> MQIELSTCFFLCLLPFCFSATRRYYLGAVELSWDYMQSDLGELHVD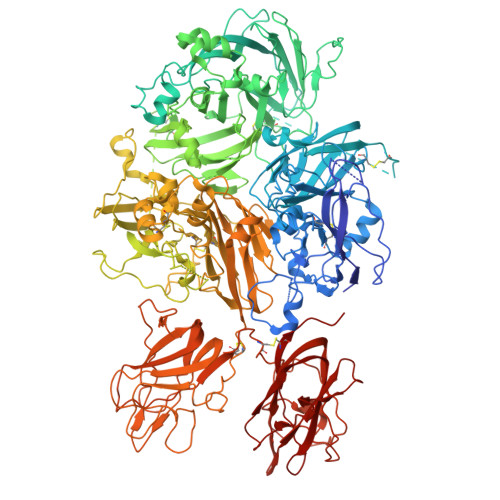TRFPPRVPKSFPFNTSVVYKKTLFVEFTDHLFNIAKPRPPWMGLLGPTIQAEVYDTVVITLKNMASHPVSLHAVGVSYWKASEGAEYDDQTSQREKEDDKVFPGGSHTYVWQVLKENGPMASDPPCLTYSYLSHVDLVKDLNSGLIGALLVCREGSLAKEKTQTLHKFILLFAVFDEGKSWHSETNNSLTQDRDAASARAQPKMHTVNGYVNRSLPGLIGCHRKSVYWHVIGMGTTPEVHSIFLEGHTFLVRNHRQASLEISPITFLTAQTLLMDLGQFLLFCHISSHQHDGMEAYVKVDSCPEEPQLRMKNNEEAEDYDDDLTDSEMDVVRFDDDNSPPFIQIRSVAKKHPKTWVHYIAAEEEDWDYAPLVLAPDDRSYKSLYLNNGPQRIGRKYKKVRFMAYTDETFKTREAIQHESGILGPLLYGEVGDTLLIIFKNQASRPYNIYPHGITDVRPLHSGRLPKGVKHLKDMPILPGEIFKYKWTVTVEDGPTKSDPRCLTRYYSSFVNLERDLASGLIGPLLICYKESVDQRGNQMMSDKRNVILFSVFDENRSWYLTENIQRFLPNPAGVQPEDPEFQASNIMHSINGYVFDSLQLSVCLHEVAYWYILSVGAQTDFLSVFFSGYTFKHKMVYEDTLTLFPFSGETVFMSMENPGLWILGCHNSDFRNRGMTALLKVSSCDKNTGDYYEDSYEDIPAYLLSKNNVIEPRSFSQNPPVLKRHQREITRTTLQPDEEKIDYDDTFSVEMKKEDFDIYGEDENQSPRSFQKKTRHYFIAAVERLWDYGMSSSPHVLRNRAQSGSVPQFKKVVFQEFTDGSFTQPLYRGELNEHLGLLGPYIRAEVEDNIMVTFKNQASRPYSFYSSLISYEEDQRQGAEPRKNFVKPNETKTYFWKVQHHMAPTKDEFDCKAWAYFSDVDLEKDVHSGLIGPLLVCRTNTLNPAHGRQVTVQEFALFFTIFDETKSWYFTENMERNCRAPCNIQMEDPTFKENYRFHAINGYIMDTLPGLVMAQDQRIRWYLLSMGSNENIHSIHFSGHVFTVRKKEEYKMALYNLYPGVFETVEMLPSKVGIWRVECLIGEHLQAGMSTLFLVYSKKCQTPLGMASGHIRDFQITASGQYGQWAPKLARLHYSGSINAWSTKEPFSWIKVDLLAPMIIHGIMTQGARQKFSSLYISQFIIMYSLDGKKWQTYRGNSTGTLMVFFGNVDSSGIKHNIFNPPIIARYIRLHPTHYSIRSTLRMELMGCDLNSCSMPLGMESKAISDAQITASSYLTNMFATWSPSQARLHLQGRSNAWRPQVNNPKEWLQVDFQKTMKVTGVTTQGVKSLLTSMYVKEFLISSSQDGHQWTLFLQNGKVKVFQGNQDSFTPVVNALDPPLLTRYLRIHPQSWAHHIALRLEVLGCEAQDLY>[2x]MFEQRVNSDVLTVSTVNSQDQVTQKPLRDSVKQALKNYFAQLNGQDVNDLYELVLAEVEQPLLDMVMQYTRGNQTRAALMMGINRGTLRKKLKKYGMN;>MYLTLQEWNARQRRPRSLETVRRWVRESRIFPPPVKDGREYLFHESAVKVDLNRP[2x]

During the site-specific DNA recombination reaction that excises phage λ from the chromosome, the bacterial DNA architectural protein Fis recruits multiple λ-encoded Xis proteins to the attR recombination site. Fis is a bacterial nucleoid protein that functions in transcription, replication, and recombination reactions. Xis is a winged-helix DNA binding protein, which is expressed at high levels shortly after prophage induction, but by itself, exhibits low binding specificity. To explore the structural basis for Fis recruitment of Xis to the X2 site within the λ prophage attR recombination site, X-ray crystal structures of three different Fis–Xis–DNA complexes were determined.

Xis was absent or was bound in an improper manner at the X1 site in our X-ray structures employing the FX1-2 sequence, even though Xis bound properly to the X2 sequence. This may be explained by the X1 sequence having an A–A (T–T) instead of a Y–R step at the 3–4 position of the Fis binding site. Thus, the native X1 sequence is incompatible with co-binding with Fis. Our three crystal structures of Fis and Xis bound to the F-X2 DNA segment reveal little (70 Å2 in the FX2 structure) or no (both FX1-2 structures) shared surface between the Xis and Fis proteins.> MNLPTAQEVQGLMARYIELVDVGDIEAIVQMFADDATVENPFGQPPIHGREQIAAFFRQGLGGGKVRACLTGPVRASHNGCGAMPFRVEMVWNGQPCALDVIDVMRFDEHGRIQTMQAFWSEVNLSVREP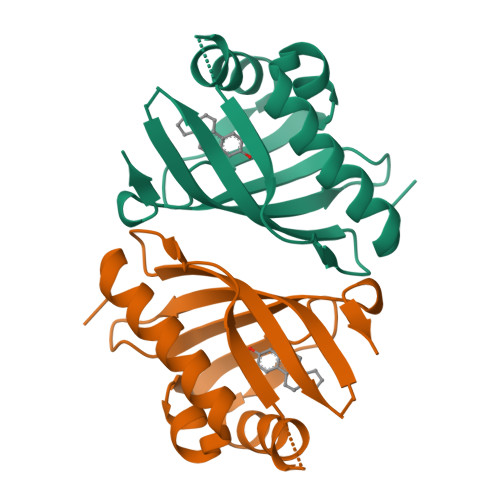Q>GSHMGSRITYVKGDLFACPKTDSLAHCISEDCRMGAGIAVLFKKKFGGVQELLNQQKKSGEVAVLKRDGRYIYYLITKKRASHKPTYENLQK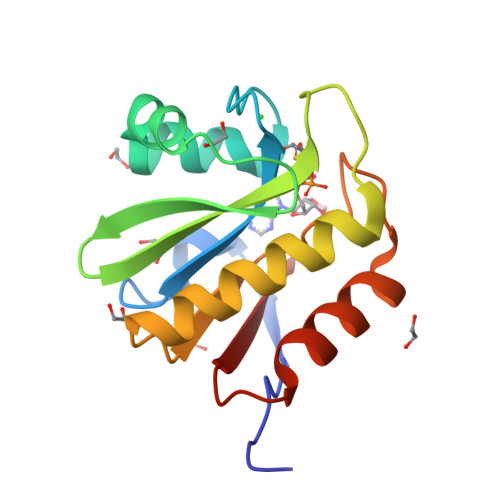SLEAMKSHCLKNGVTDLSMPRIGCGLDRLQWENVSAMIEEVFEATDIKITVYTL[4x]>GPGSMTDAPGALAERRGNVMVITINRPEARNAINAAVSIGVGDALEEAQHDPEVRAVVLTGAGDKSFCAGADLKAIARRENLYHPDHPEWGFAGYVRHFIDKPTIAAVNGTALGGGTELALASDLVVADERAQFGLPEVKRGLIAAAGGVFRIAEQLPRKVAMRLLLTGEPLSAAAARDWGLINEVVEAGSVLDAALALASAITVNAPLSVQASKRIAYGVDDGVVVGDEPGWDRTMRE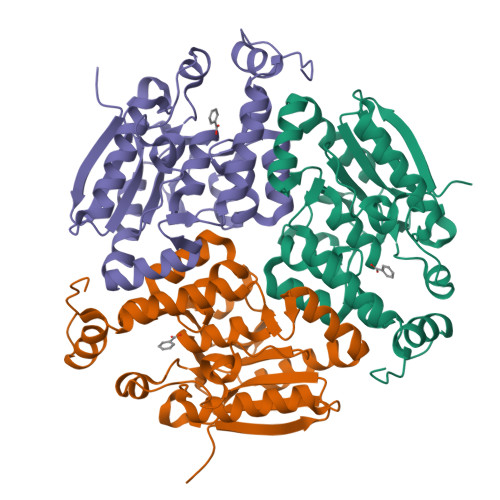MRALLKSEDAKEGPRAFAEKREPVWQAR[3x]To investigate the photophysics of special pairs independently of the complexities of native photosynthetic proteins, and as a first step toward creating synthetic photosystems for new energy conversion technologies, we designed C2-symmetric proteins that hold two chlorophyll molecules in closely juxtaposed arrangements. For Chl dimer protein scaffolds, we chose hyperstable C2-symmetric repeat protein dimers containing symmetric pockets with tunable sizes and geometries. In this dimeric repeat protein architecture, the hydrophobic core is independent of the small molecule-binding site, enabling full customization for binding with little impact on the overall protein structure. We describe de novo-designed proteins that hold Chl dimers in precisely defined, closely juxtaposed geometries.

We did not succeed in solving the holo-state structure of SP3; however, we were able to solve a 3.05 Å-resolution apo-state structure of the closely related design SP3x, which shares 94% sequence identity with SP3. The SP3x homodimeric design model agrees with the X-ray crystal structure to 1.61 Å Cα r.m.s.d. In the SP3 dimer, the calculated spectrum based on the design model agreed with the experimentally measured signs of the CD Cotton effects, suggesting that the P700-like ZnPPaM dimer in SP3 assembles as designed.

>SGSSEELARESAEAAWRLAQASTRATLAMIRGDLKELAEALIELARAVQELARVAKEYGNDELAKTAALLAAHVAMLAIWVLIRAIKEGDDEVRELAKTAIKLASTAAKIVLDALPTAEEVRQITLLAKLAEEAADKKNEDSALAVGIAAIAVIIALWALEAAQKAGIEEAEKGARLLLKLAMDAARKKNPEEALAVLNAALDVSIALQLLQSAKRAGSEETRKLAEEMLRQALERARKKN[2x]> MAAGQNGHEEWVGSAYLFVESSLDKVVLS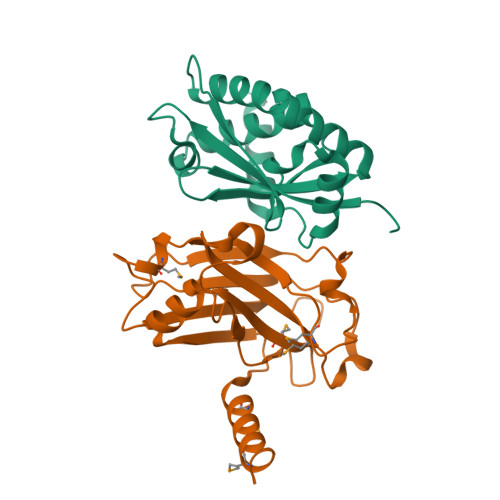DAYAHPQQKVAVYRALQAALAESGGSPDVLQMLKIHRSDPQLIVQLRFCGRQPCGRFLRAYREGALRAALQRSLAAALAQHSVPLQLELRAGAERLDALLADEERCLSCILAQQPDRLRDEELAELEDALRNLKCGSGARGGDGEVASAP;> KDLAMADLEQKVLEMEASTYDGVFIWKISDFPRKRQEAVAGRIPAIFSPAFYTSRYGYKMCLRIYLNGDGTGRGTHLSLFFVVMKGPNDALLRWPFNQKVTLMLLDQNNREHVIDAFRPDVTSSSFQRPVNDMNIASGCPLFCPVSKMEAKNSYVRDDAIFIKAIVDLTGL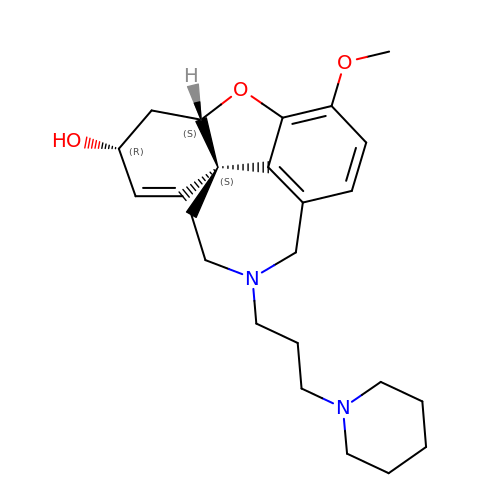(4aS,6R,8aS)-3-methoxy-11-(3-piperidin-1-ylpropyl)-5,6,9,10,11,12-hexahydro-4aH-[1]benzofuro[3a,3,2-ef][2]benzazepin-6-ol | C24 H34 N2 O3 | JIMPGPISVDHAIE-PTLVVNQVSA-N>[2x]MGGSHHHHHHLESTSLYKKSSSTPPRGVTVVNNFDCKRYLGTWYEIARFDHRAERGLEKVTATYSLRDDGGLNVIFKGYNPDRGMWQQYVGKAYFTGAPTRAALKVAFFGPFYG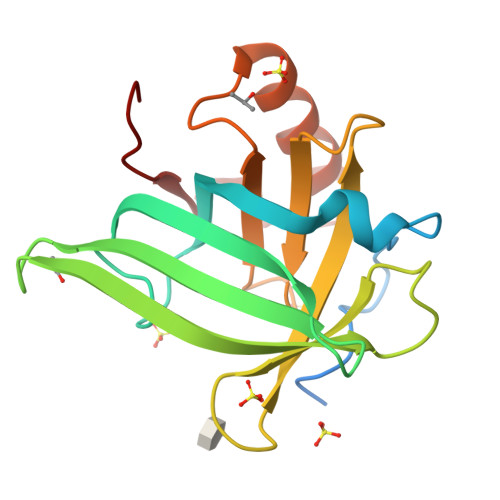GYNVIALDREYRHALVCGPDRDYLWINSRTPTISDEVKQEMLAVATREGFDVSKFIWVQQPGS>SGTVKYTDAQIQRLREYGNGTYEQKVFEDLASRDAAFSKEMSVASTDNEKKIKGMIANPSRHGLTQLMNDIADALVAEGFIEVRTPIFISKDALARMTITEDKPLFKQVFWIDEKRALRPMLAPNLYSVMRDLRDHTDGPVKIFEMGSCFRKESHSGMHLEEFTMLALGDMGPRGDATEVLKNYISVVMKAAGLPDYDLVQEESDVYKETIDVEINGQEVCSAAVGPHYLDAAHDVHEPCSGAGFGLERLLTIREKYSTVKKGGASISYLNGAK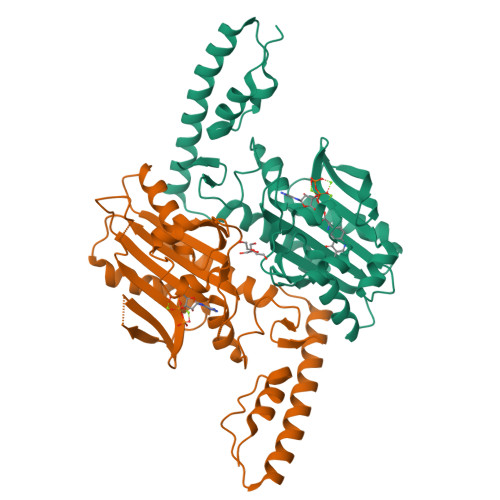IN[2x]> MVSVINTVDTSHEDMIHDAQMDYYGIRLATCSSDRSVKIFDVKNGGQILIADLRGHDGPVWQVAWAHPMYGNILASCSYDRKVIIWKEENGTWEKTYEYTGHDSSVNSVCWAPHDFGLVLACGSSDGAISILTFTGDGPWEVKKISNAHTIGCNAVSWAPSVIPGSLVDQPSSQKPNYIKRFVSGGCDNLVKIWREEDGQWKEDQKLEAHSDWVRDVAWAPSIGLPTSTIASCSQDGRVYIWTSDDAATNCWTPKLLHKFNDVVWHVSWSITANILAVSGGDNKVT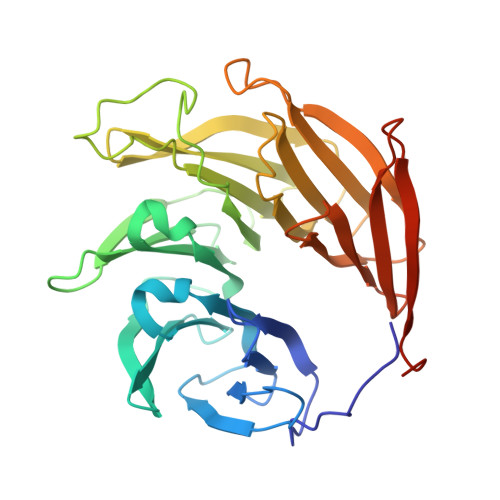LWKESVDGQWACISDVNKGQGAVSTVTEGQLNDQ>MGSSHHHHHHSSGMNRHTDTHYPSLADKVVLISGGASGIGRAFVEAFVAQGSRVAFLDLDAEAGQGLAHALGANSLFLPCDVRDIERLKACVAEVERTWGAVDVLINNAARDDRHALADVSVEYWDERMQTNLRHAFFAAQAVAPGMARRGSGAIINMGSISWMRGRPGMVCYTTAKAALNGMTRTLARELGGQGIRINSLVPGAIRTERQDAMWAADPAGLEAASQAFIDQQMLKFRLDASDCARLALFLASDDSRGCTGQNFVVDAGLSIQ[2x]

The sulfosugar sulfoquinovose (SQ) is catabolized through the sulfoglycolytic Entner-Doudoroff pathway, beginning with the oxidation of SQ to sulfogluconolactone by SQ dehydrogenase. PpSQDH is a tetrameric enzyme belonging to the short-chain dehydrogenase/reductase (SDR) superfamily with a strong preference for NAD+ over NADP+. Kinetic analysis revealed a rapid equilibrium ordered mechanism in which the NAD+ cofactor is the first substrate to bind, and NADH is the last product to dissociate. Structural studies revealed a homotetrameric structure in solution and crystals, involving cross-subunit interactions in which the C-terminus residue (Gln260) inserts into the diagonally opposite subunit to form part of the second shell of residues lining the active site.

To elucidate the enzyme-substrate interactions of PpSQDH, 3D X-ray crystal structures of apo-PpSQDH as well as binary complexes of PpSQDH•NAD+ and PpSQDH•SQ were obtained to resolutions of 1.7, 1.9 and 1.9 Å, respectively, each in the I2 space group with two molecules in the asymmetric unit. Size exclusion chromatography-multi angle laser light scattering (SEC-MALLS) analysis detected a dominant solution state species of ~119 kDa (monomer molecular weight of 28,000 Da, confirmed by LC-MS analysis), thereby demonstrating a tetrameric assembly of PpSQDH in solution as commonly seen for members of the SDR family. PISA (Proteins Interfaces, Surface & Assemblies) analysis shows that the compact tetrameric assembly of PpSQDH subunits buries a total of 13,974 Å2 of solvent-accessible surface area, which accounts for 29% of the total surface area of the oligomer. PpSQDH adopts the classical SDR fold with a highly conserved active site architecture comprising the Asn119-Ser147-Tyr160-Lys164 catalytic tetrad. Each subunit consists of an N-terminal Rossmann fold with a central, parallel β-sheet (β1–7) sandwiched by α helices on either side, followed by a smaller C-terminal region. We observe an ordered region with a higher B-factor (residues 195–218) in the crystal structure of ligand-free PpSQDH close to the C-terminal end, which corresponds to the extensively documented substrate-binding loop of SDR dehydrogenases.> MAKTVILDHDGNKDDFVAMILLLSNPKKVNLIGCICTDADCFVENGFDVTGKIMCAMHRLIKTPLFPIGKSTATAVNAFPTEWRFSAKNLDDMPFLNIVEDVALWEKLKPENEAHNGQQLLADLVMKSKEKVTVCVTGPLSNMAWCIEKYGEAFTSKVEECVIMGGAVDVGGNVFLPTTDGSAEWNIYWDPPAAKKVLCCPNIRCVLFSLDATNTVPVRSVDVKGFGAQN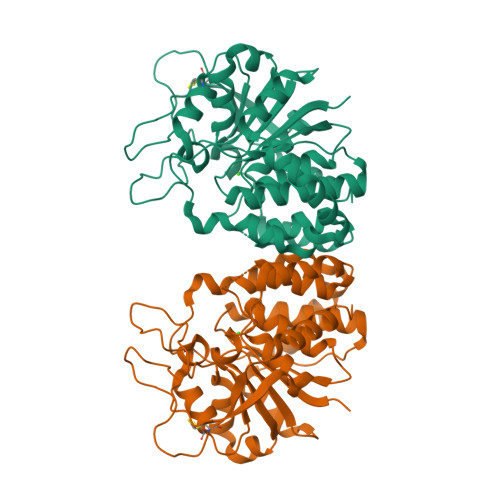QYLLSQMVGTMWAMSTHEEILRDGDAYYAWDALTAAYILEPTIATLEPVALDVDVSKGKSEGRTPRASGEGKPCVHVARNPSKQMFHDLVFASTRVC Mutations in CK1δ/ε (hereafter referred to jointly as CK1), as well as PER2, exert powerful control over circadian period, altering the intrinsic timing of circadian rhythms by hours in vivo. PER2 is regulated by a CK1-dependent phosphoswitch, where kinase activity at two antagonistic sites functionally interact to control PER2 stability. We discovered a conformational switch in the activation loop of CK1 that regulates its activity on two regulatory regions in PER2 that control its stability and circadian timing in mammals. We show that anion binding regulates the conformation of this switch to reshape the substrate binding cleft and thereby control substrate selectivity.

To test the role of Site 2 anion binding in regulation of CK1 activity, we made charge reversion mutants at positions R127 and K154, as well as at K171 located nearby on the activation loop, and measured enzymatic efficiency (kcat/Km) on FASP and Degron peptides in vitro. We observed a modest decrease (~25%) in activity towards the FASP peptide, suggesting that the ‘loop down’ conformation that is enforced by anion binding at Site 2 may be important for FASP activity. Strikingly, these mutants all increased activity towards the Degron, with a ~ 50% gain in efficiency for R127E. To further examine the role of K171 in regulation of anion binding, we solved a structure of the K171E mutant crystallized in high sulfate conditions and found a full complement of three anions bound, demonstrating that local flexibility in the activation loop allows it to retain sulfate binding at Site 2 to some degree. Overall, these data suggest that anion binding at Site 2 correlates with substrate selectivity on the FASP and Degron peptides. Notably, the change in selectivity with Site 2 mutants in vitro makes them much more tau-like, consistent with a recent report that both tau and charge reversion mutants at Site 2 lead to decreased PER2 stability in cells.

>MELRVGNRYRLGRKIGSGSFGDIYLGTDIAAGEEVAIKLECVKTKHPQLHIESKIYKMMQGGVGIPTIRWCGAEGDYNVMVMELLGPSLEDLFNFCSRKFSLKTVLLLADQMISRIEYIHSKNFIHRDVKPDNFLMGLGKKGNLVYIIDFGLAKKYRDARTHQHIPYRENENLTGTARYASINTHLGIEQSRRDDLESLGYVLMYFNLGSLPWQGLKAATKRQKYERISEKKMSTPIEVLCKGYPSEFATYLNFCRSLRFDDKPDYSYLRQLFRNLFHRQGFSYDYVFDWNMLK[2x]>MGSLPCDICKDVVTAAGDMLKDNATEEEILVYLEKTCDWLPKPNMSASCKEIVDSYLPVILDII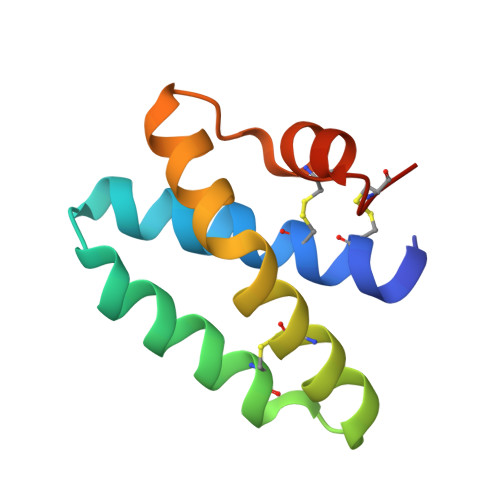KGEMSRPGEVCSALNLCESLQ[2x]>QPQFNEDTLQQRLQALIESAGENWTYAIFWQISHDFDSSTGDNTVILGWGDGYYKGEEDKEKKKNNTNTAEQEHRKRVIRELNSLISGGIGVSDESNDEEVTDTEWFFLVSMTQSFVNGV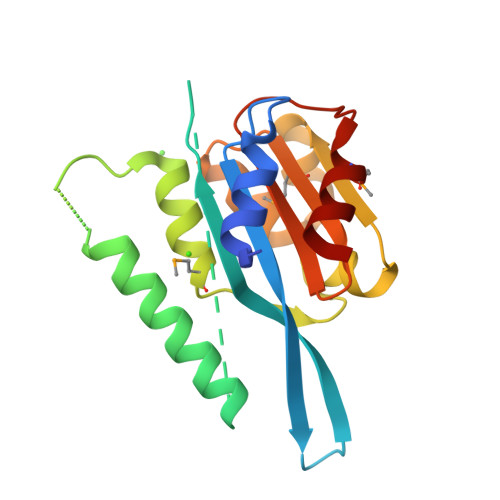GLPGESFLNSRVIWLSGSGALTGSGCERAGQGQIYGLKTMVCIATQNGVVELGSSEVISQSSDLMHKVNNLFNFN[2x]> GSHMEFMAEQATKSVLFVCLGNICRSPIAEAVFRKLVTDQNISENWRVDSAATSGYEIGNPPDYRGQSCMKRHGIPMSHVARQ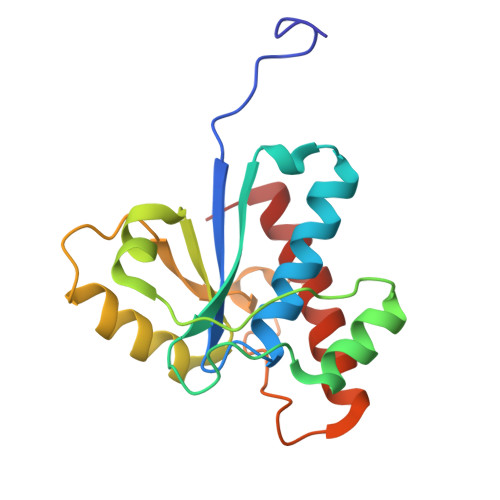ITKEDFATFDYILCMDESNLRDLNRKSNQVKTCKAKIELLGSYDPQKQLIIEDPYYGNDSDFETVYQQCVRCCRAFLEKAH>[2x]MPAPQDPRNLPIRQQMEALIRRKQAEITQGLESIDTVKFHADTWTRGNDGGGGTSMVIQDGTTFEKGGVNVSVVYGQLSPAAVSAMKADHKNLRLPEDPKTGLPVTDGVKFFACGLSMVIHPVNPHAPTTHLNYRYFETWNQDGTPQTWWFGGGADLTPSYLYEEDGQLFHQLHKDALDKHDTALYPRFKKWCDEYFYITHRKETRGIGGIFFDDYDERDPQEILKMVEDCFDAF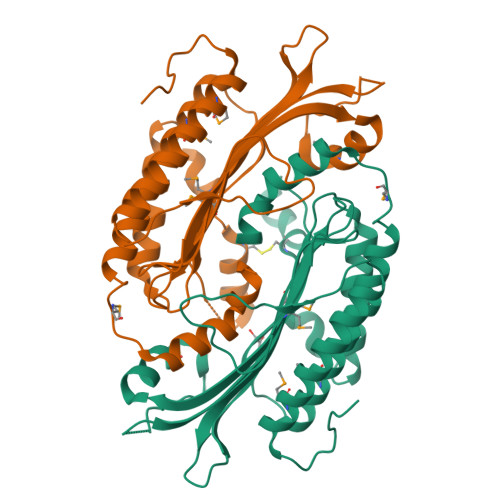LPSYLTIVKRRKDMPYTKEEQQWQAIRRGRYVEFNLIYDRGTQFGLRTPGSRVESILMSLPEHASWLYNHHPAPGSREAKLLEVTTKPREWVK4-[2-(5,5,8,8-tetramethyl-6,7-dihydroquinoxalin-2-yl)ethynyl]benzoic 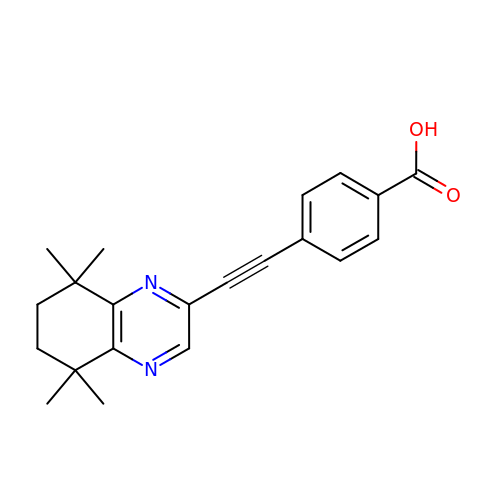acid | C21 H22 N2 O2 | BUYUFJZVMVFQLQ-UHFFFAOYSA-N>TPKPKIVLVGSGMIGGVMATLIVQKNLGDVVMFDVVKNMPQGKALDTSHSNVMAYSNCKVTGSNSYDDLKGADVVIVTAGFTKAPGKSDKEWNRDDLLPLNNKIMIEIGGHIKNLCPNAFIIVVTNPVDVMVQLLFEHSGVPKNKIIGLGGVLDTSRLKYYISQKLNVCPRDVNALIVGAHGNKMVLLKRYITVGGIPLQEFINNKKITDEEVEGIFDRTVNTALEIVNLLASPYVAPAAAIIEMAESYLKDIKKVLVCSTLLEGQYGHSNIFGGTPLVIGGTGVEQVIELQLNAEEKTKFDEAVAETKRMKALIHHH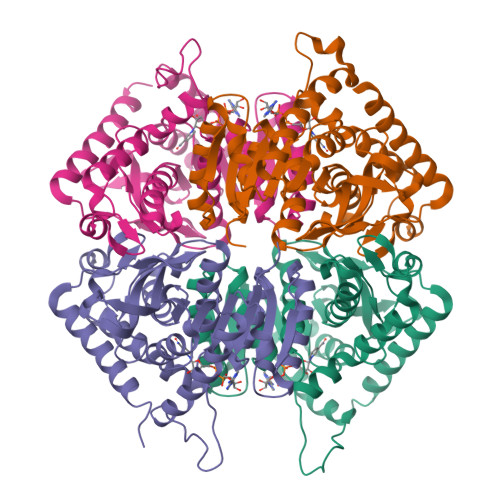HHH[4x]> SNLKIVRMDRTAGCVTGGE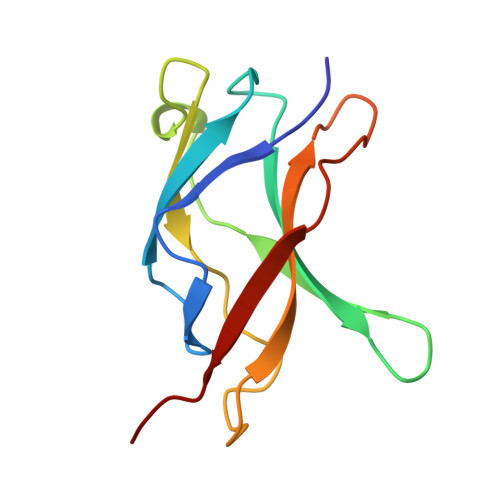EIYLLCDKVQKDDIQIRFYEEEENGGVWEGFGDFSPTDVHRQFAIVFKTPKYKDINITKPASVFVQLRRKSDLETSEPKPFLYYPEIK>[2x]MKILFVASGSPATVFALAPLATAARNAGHDVFMGAVEDMVPYIASAGIPALSIAPSSIRRYATMDREGNPVRMPETPEEELDFAGHWFGRMAAGSMDALREVTANWRPDLVVGGSMSFAAALIAAELGVPYVRQAWDTGDAWRTDPAASDELRPELRALGLDRLPDPALFVDICPPSLRPATAPPAQMMRWVPANGQRRLEPWMYTKGNRPRILVTSGSRLVFAKKTGFLRGLVADMAALDA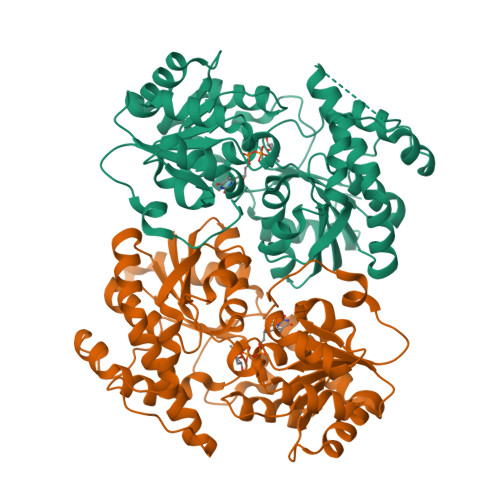EVVIATLDEVAEELRTELPGVRAGWVPLDVVVPTCDVVVHHAGGVTALTAMNAGVPQLIVPQGGNFVEAGLRISDFGAAITVDENTPEAVEKACGELIGNPSYAERARELSAEIAALPLPAEVVGALEGLVENLYFQ>LVSSPSTLNPGTNVAKLAEQAPVHWVSVAQIENSLTGRPPMAVGFDIDDTVLFSSPGFWRGKKTYSPDSDDYLKN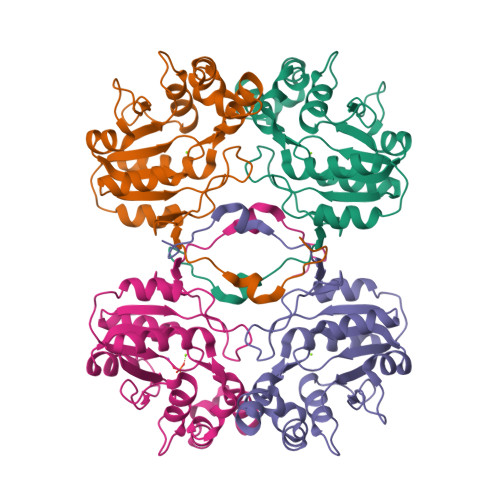PAFWEKMNNGWDEFSIPKEAARQLIDMHVRRGDSIYFVTGRSQTKTETVSKTLADNFHIPAANMNPVIFAGDKPEQNTNVQWLQEKNMRIFYGDSDNDITAARDCGIRGIRILRAANSTYKPLPQAGAFGEEVIVNSEY[4x]>GAMEDENILRNAVNLQVLKFHYPEIESIIDIASHVAVYQFDVGSQKWLKTSIEGTFFLVKDQRARVGYVILNRNSPENLYLFINHPSNVHLVDRYLIHRTENQHVVGLWMFDPNDMSRIFNIVKESLLR[2x];>[2x]MGMSFTNATFSQVLDDLSARFILNLPAEEQSSVERLCFQIEQAHWFYEDFIRAQNDQLPSLGLRVFSAKLFAHCPLLWKWSKVHEEAFDDFLRYKTRIPVRGAIMLDMSMQQCVLVKGWKASSGWGFPKGKIDKDESDVDCAIREVYEETGFDCSSRINPNEFIDMTIRGQNVRLYIIPGISLDTRFESRTRKEISKIEWHNLMDLPTFKKNKPQT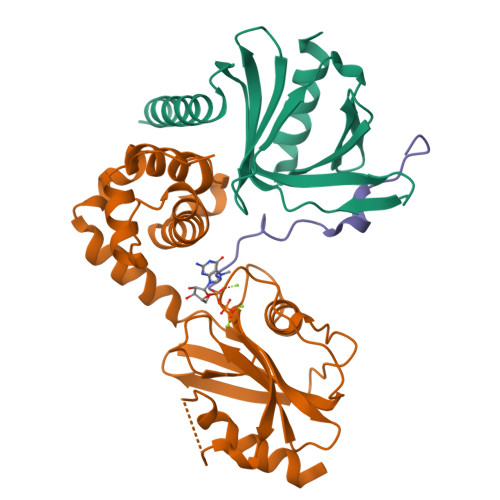MKNKFYMVIPFLAPLKKWIKKRNIANNTT;>[2x]SILYAGPTFTHSPAASNLPIPTFLHS> GFFQLFRFSSSTDIWLMFVGSLCAFLHGIAQPGVLLIFGTMTDVFIDYDVELQELQIPGKACVNNTIVWTNSSLNQNMTNGTRCGLLNIESEMIKFASYYAGIAVAVLITGYIQICFWVIAAARQIQKMRKFYFRRIMRMEIGWFDCNSVGELNTRFSDDINKINDAIADQMALFIQRMTSTICGFLLGFFRGWKLTLVIISVSPLIGIGAATIGLSVSKFTDYELKAYAKAGVVADEVISSMRTVAAFGGEKREVERYEKNLVFAQRWGIRKGIVMGFFTGFVWCLIFLCYALAFWYGSTLVLDEGEYTPGTLVQIFLSVIVGALNLGNASPCLEAFATGRAAATSIFETIDRKPIIDCMSEDGYKLDRIKGEIEFHNVTFHYPSRPEVKILNDLNMVIKPGEMTALVGPSGAGKSTALQLIQRFYDPCEGMVTVDGHDIRSLNIQWLRDQIGIVEQEPVLFSTTIAENIRYGREDATMEDIVQAAKEANAYNFIMDLPQQFDTLVGEGGGQMSGGQKQRVAIARALIRNPKILLLDMATSALDNESEAMVQEVLSKIQHGHTIISVAHRLSTVRAADTIIGFEHGTAVERGTHEELLERKGVYFTLVTLQSQGNQALNEEDIKDATEDDMLARTFSRGSYQDSLRASIRQRSKSQLSYLVHEPPLAVVDHKSTYEEDRKDKDIPVQEEVEPAPVRRILKFSAPEWPYMLVGSVGAAVNGTVTPLYAFLFSQILGTFSIPDKEEQRSQINGVCLLFVAMGCVSLF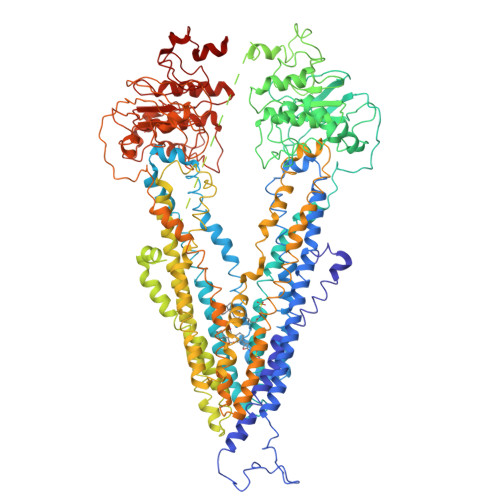TQFLQGYAFAKSGELLTKRLRKFGFRAMLGQDIAWFDDLRNSPGALTTRLATDASQVQGAAGSQIGMIVNSFTNVTVAMIIAFSFSWKLSLVILCFFPFLALSGATQTRMLTGFASRDKQALEMVGQITNEALSNIRTVAGIGKERRFIEALETELEKPFKTAIQKANIYGFCFAFAQCIMFIANSASYRYGGYLISNEGLHFSYVFRVISAVVLSATALGRAFSYTPSYAKAKISAARFFQLLDRQPPISVYNTAGEKWDNFQGKIDFVDCKFTYPSRPDSQVLNGLSVSISPGQTLAFVGSSGCGKSTSIQLLERFYDPDQGKVMIDGHDSKKVNVQFLRSNIGIVSQEPVLFACSIMDNIKYGDNTKEIPMERVIAAAKQAQLHDFVMSLPEKYETNVGSQGSQLSRGEKQRIAIARAIVRDPKILLLDEATSALDTESEKTVQVALDKAREGRTCIVIAHRLSTIQNADIIAVMAQGVVIEKGTHEELMAQKGAYYKLVT> KEAMGHMQEVVDGLWVGDLVAANDDDELEKNGIKNILSALRPSLKFSDKYAVYPLEI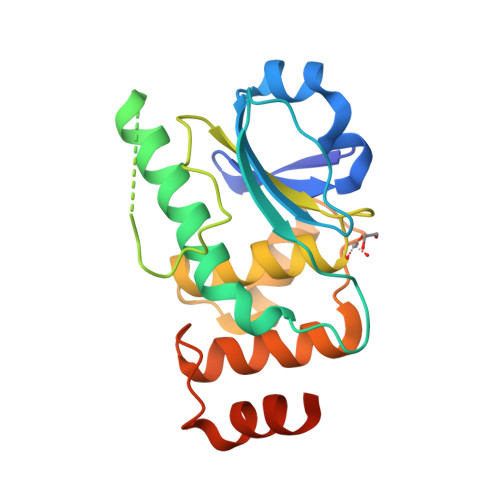DDSADTDLLSHLPSCVAWIKEILDLRQKAAEPSSQKNGTENGESLKRSPDIDTVAQPGKPGGVLVHCQAGMSRSASIVAAYLMSQYDLDPMEAMTMIREKRPVVEPSATFWHQLGLFYTTDGKVSLKDRSTRQYYMERTTTQFINGDG>MTSVNSAEASTGAGGGGSNPVKSMWSEGATFSANSVTCTFSRQFLIPYDPEHHYKVFSPAASSCHNASGKEAKVCTISPIMGYSTPWRYLDFNALNLFFSPLEFQHLIENYGSIAPDALTVTISEIAVKDVTDKTGGGVQVTDSTTGRLCMLVDHEYKYPYVLGQGQDTLAPELPIWVYFPPQYAYLTVGDVNTQGISGDSKKLASEESAFYVLEHSSFQLLGTGGTATMSYKFPPVPPENLEGCSQHFYEMYNPLYGSRLGVPDTLGGDPKFRSLTHEDHAIQPQNFMPGPLVNSVSTKEGDSSNTGAGKALTGLSTGTSQNTRISLRPGPVSQPYHHWDTDKYVTGINAISHGQTTYGNAEDKEYQQGVGRFPNEKEQLKQLQGLNMHTYFPNKGTQQYTDQIERPLMVGSVWNRRALHYESQLWSKIPNLDDSFKTQFAALGGWG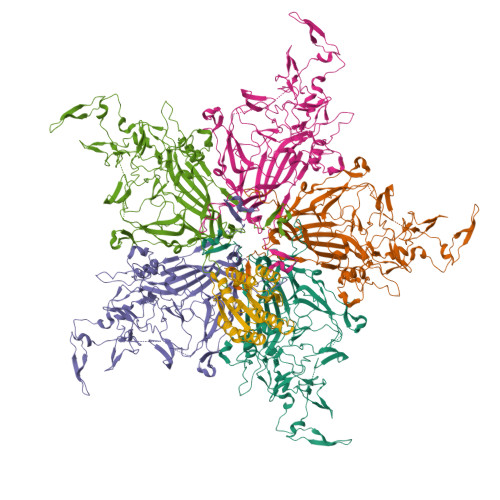LHQPPPQIFLKILPQSGPIGGIKSMGITTLVQYAVGIMTVTMTFKLGPRKATGRWNPQPGVYPPHAAGHLPYVLYDPTATDAKQHHRHGYEKPEELWTAKSRVHPL[5x];> MKPPRPVRTCSKVLVLLSLLAIHQTTTAEKNGIDIYSLTVDSRVSSRFAHTVVTSRVVNRANTVQEATFQMELPKKAFITNFSMIIDGMTYPGIIKEKAEAQAQYSAAVAKGKSAGLVKATGRNMEQFQVSVSVAPNAKITFELVYEELLKRRLGVYELLLKVRPQQLVKHLQMDIHIFEPQGISFLETESTFMTNQLVDALTTWQNKTKAHIRFKPTLSQQQKSPEQQETVLDGNLIIRYDVDRAISGGSIQIENGYFVHYFAPEGLTTMPKNVVFVIDKSGSMSGRKIQQTREALIKILDDLSPRDQFNLIVFSTEATQWRPSLVPASAENVNKARSFAAGIQALGGTNINDAMLMAVQLLDSSNQEERLPEGSVSLIILLTDGDPTVGETNPRSIQNNVREAVSGRYSLFCLGFGFDVSYAFLEKLALDNGGLARRIHEDSDSALQLQDFYQEVANPLLTAVTFEYPSNAVEEVTQNNFRLLFKGSEMVVAGKLQDRGPDVLTATVSGKLPTQNITFQTESSVAEQEAEFQSPKYIFHNFMERLWAYLTIQQLLEQTVSASDADQQALRNQALNLSLAYSFVTPLTSMVVTKPDDQEQSQVAEKPMEGESRNRNVHSGSTFFKYYLQGAKIPKPEASFSPRRGWNRQAGAAGSRMNFRPGVLSSRQLGLPGPPDVPDHAAYHPFRRLAILPASAPPATSNPDPAVSRVMNMKIEETTMTTQTPAPIQAPSAILPLPGQSVERLCVDPRHRQGPVNLLSDPEQGVEVTGQYEREKAGFSWIEVTFKNPLVWVHASPEHVVVTRNRRSSAYKWKETLFSVMPGLKMTMDKTGLLLLSDPDKVTIGLLFWDGRGEGLRLLLRDTDRFSSHVGGTLGQFYQEVLWGSPAASDDGRRTLRVQGNDHSATRERRLDYQEGPPGVEISCWSVEL> MWSHPQFEKENLYFQGIYISAVGMLNALGDNVDDIAQNLVLGQAPGMYERSGWLQPGKTCCLGGVDAELPAMPDMLSEHNSRNNRLLLAALMQIKPQVDEAIARHGRERIAVIMGTSTSGLDEGDQHVSRTVYQQSHGSYHDYHYYQQELGDPSRFLARYLAIEGPAFTLSTACSSSSRAIISGQRLIEMGLVDAAIVGGADTLSRMPINGFDSLESLSPTLCEPFCQDRQGITIGEASTLLLLTREPQPIALLGVGESSDAWHMSAPHPEGRGAIAAI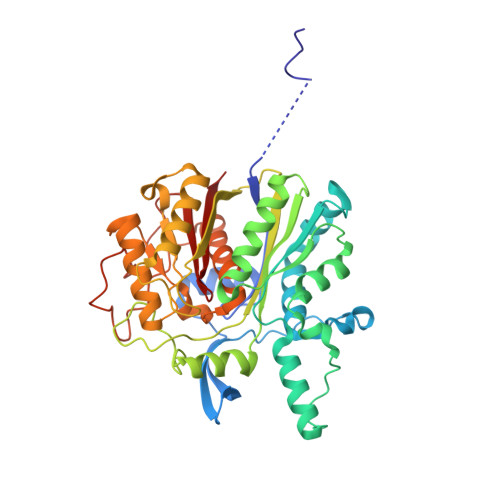NMALRKAGISPAEIGYINLHGTGTKLNDQMESIVINQIFGENTPCSSTKYLTGHTLGAAGACEAGLCWLLLTRHLPLPAQDFTRSGIDIALPACGLLTQSQPLEKPIVMSNSFAFGGNNTSLILGVA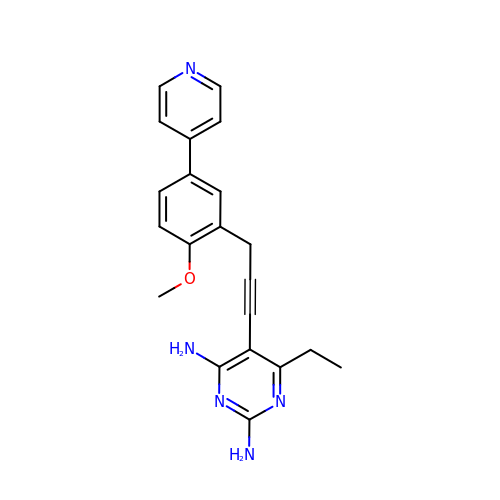6-ethyl-5-{3-[2-methoxy-5-(pyridin-4-yl)phenyl]prop-1-yn-1-yl}pyrimidine-2,4-diamine | C21 H21 N5 O | CZCHMGRCEXJPTP-UHFFFAOYSA-N>[2x]MQLTKCEVFQKLKDLKDYGGVSLPEWVCTAFHTSGYDTQAIVQNNDSTEYGLFQINNKIWCK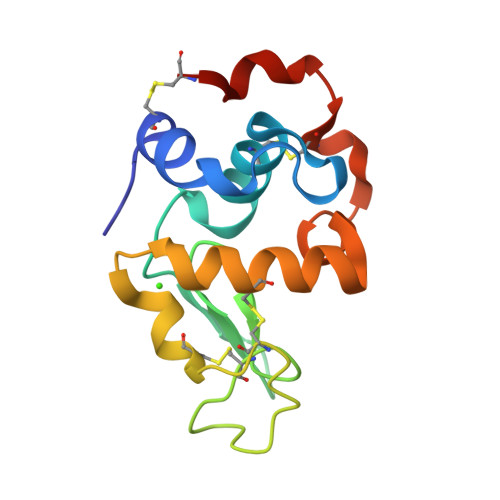DDQNPHSRNICNISCDKFLDDDLTDDIVCAKKILDKVGINYWLAHKALCSEKLDQWLCEKL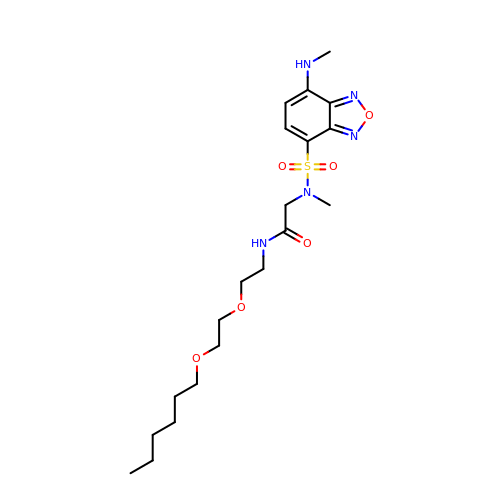N-{2-[2-(hexyloxy)ethoxy]ethyl}-N~2~-methyl-N~2~-{[7-(methylamino)-2,1,3-benzoxadiazol-4-yl]sulfonyl}glycinamide | C20 H33 N5 O6 S | BINKCYCULJAFGO-UHFFFAOYSA-N> MWFFNKNLKVLAPCDGTIITLDEVEDEVFKERMLGDGF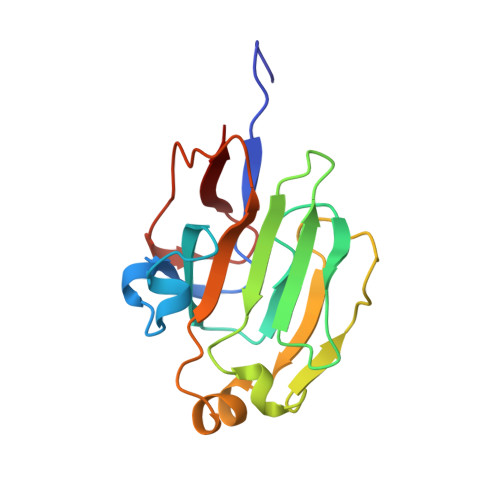AINPKSNDFHAPVSGKLVTAFPTKHAFGIQTKSGVEILLHIGLDTVSLDGNGFESFVTQDQEVNAGDKLVTVDLKSVAKKVPSIKSPIIFTNNGGKTLEIVKMGEVKQGDVVAILK>MALFVRLLALALALALGPAATLAGPAKSPYQLVLQHSRLRGRQHGPNVCAVQKVIGTNRKYFTNCKQWYQRKICGKSTVISYECCPGYEKVPGEKGCPAALPLSNLYETLGVVGSTTTQLYTDRTEKLRPEMEGPGSFTIFAPSNEAWASLPAEVLDSLVSNVNIELLNALRYHMVGRRVLTDELKHGMTLTSMYQNSNIQIHHYPNGIVTVNCARLLKADHHATNGVVHLIDKVISTITNNIQQIIEIEDTFETLRAAVAASGLNTMLEGNGQYTLLAPTNEAFEKIPSETLNRILGDPEALRDLLNNHILKSAMCAEAIVAGLSVETLEGTTLEVGCSGDMLTINGKAIISNKDILATNGVIHYIDELLIPDSAKTLFELAAESDVSTAIDLFRQAGLGNHLSGSERLTLLAPLNSVFKDGTPPIDAHTRNLLRNHIIKDQLASKYLYHGQTLETLGGKKLRVFVYRNSLCIENSCIAAHDKRGRYGTLFTMDRVLTPPMGTVMDVLKGDNRFSMLVAAIQSAGLTET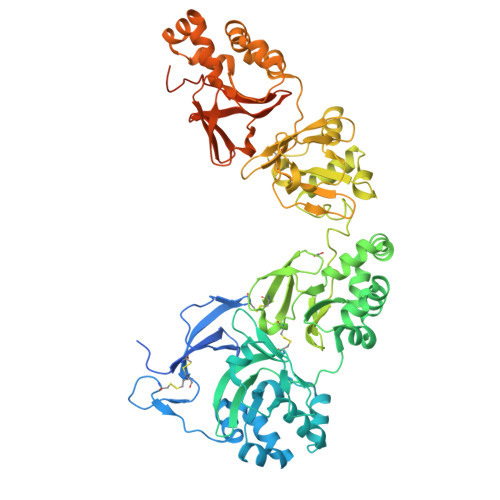LNREGVYTVFAPTNEAFRALPPRERSRLLGDAKELANILKYHIGDEILVSGGIGALVRLKSLQGDKLEVSLKNNVVSVNKEPVAEPDIMATNGVVHVITNVLQPPANRPQERGDELADSALEIFKQASAFSRASQRSVRLAPVYQKLLERMKH[2x]>[4x]MSNEIPKPVAPAPDILRCAYAELVVTDLAKSRNFYVDVLGLHVSYEDENQIYLRSFEEFIHHNLVLTKGPVAALKAMAFRVRTPEDVDKAEAYYQELGCRTERRKDGFVKGIGDALRVEDPLGFPYEFFFETTHVERLHMRYDLYSAGELVRLDHFNQVTPDVPRGRKYLEDLGFRVTEDIQDDEGTTYAAWMHRKGTVNDTALTGGNGPRLHHVAFSTHEKHNIIQICDKMGALRIS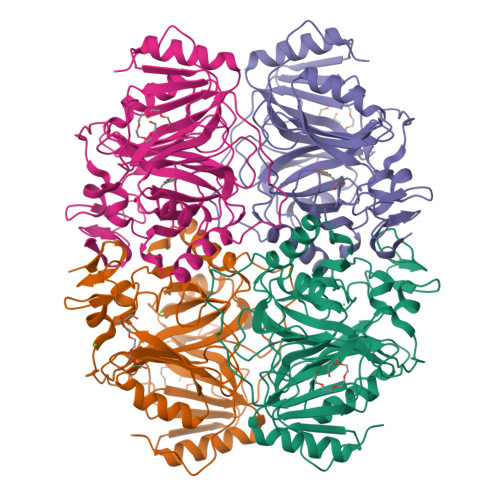DRIERGPGRHGVSNAFYLYILDPDNHRIEIYTQDYYTGDPDNPTITWNVHDNQRRDWWGNPVVPSWYTEASKVLDLDGNVQEIIERTDDSELEVTIGADGFSFTRAGDEDGSYHGQASKGFKLGNQL> IVGGRKARPRQFPFLASIQNQGSHECGGALIHARFVMTAASCFQSQ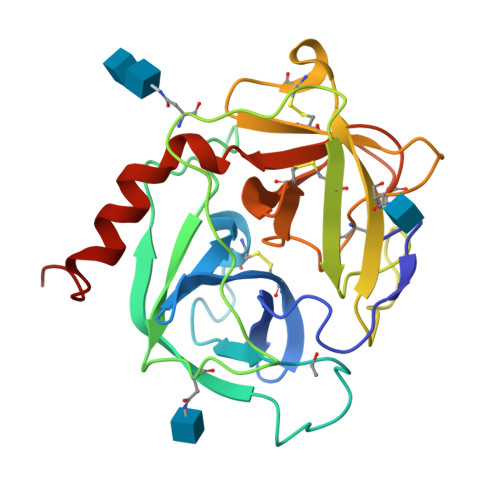NPGVSTVVLGAYDLRRRERQSRQTFSISSMSENGYDPQQNLNDLMLLQLDREANLTSSVTILPLPLQNATVEAGTRCQVAGWGSQRSGGRLSRFPRFVNVTVTPEDQCRPNNVCTGVLTRRGGICNGDGGTPLVCEGLAHGVASFSLGPCGRGPDFFTRVALFRDWIDGVLNNPGPGPA>GSHMESFLLSKVSFVIKKIRLEKGMTQEDLAYKSNLDRTYISGIERNSRNLTIKSLELIMKGLEVSDVVFFEMLIKEILKHD[2x]

The most widespread of these mechanisms employs a “controller” (C) protein encoded by a gene downstream of its own promoter, and usually co-transcribed with the endonuclease (R) gene as a single transcriptional unit. The C-protein binds at various sites within the C/R promoter to regulate transcription of its own gene and the associated endonuclease gene. Unusually, in the RM system Esp1396I, the C-protein also represses the MTase (M) gene by binding to the promoter at the transcriptional start site, denoted OM where the C/R genes and the M gene are transcribed convergently from different promoters. Flexibility in this loop is very important for DNA sequence recognition, as it has been observed in the nucleoprotein structures to adopt different conformations depending on which operator site the protein is bound to.

Since the resolution of the diffraction data from each mutant protein (1.5–2.0 Å) was significantly better than the previously determined native structure (2.7 Å), we also crystallized the native protein and obtained crystals that diffracted to much higher resolution (1.4 Å) than the published structure, to permit a more accurate comparison. Overall the new triclinic wild type and mutant protein structures closely resemble the original protein structure. One obvious feature of the higher resolution structures was the presence of several water molecules on the surface of the proteins. The side chain positions could also be placed with a higher degree of confidence. In terms of crystal contacts, Y29 does not stack with a symmetry related Y29 residue in the manner observed in several C.Esp1396I crystal structures. A large number of crystal contacts occur through the C-terminal tail of C.Esp1396I and symmetry related chains. This gives that previously flexible region a high degree of stability, allowing the complete C-terminus up to the terminal carboxyl oxygen atoms to be modelled. The other primary intermolecular interface is centred on one of the SO4 ions. The SO4 ion essentially bridges the gap between symmetry related chains as in this region no direct protein-protein interactions occur. The wild type structure of C.Esp1396I presented in this study revealed further details including an additional, third conformation of the flexible loop region that was subsequently observed in several of the mutant protein structures.> MHHHHHHSEINPAEFEQVNMVLQGFVETSVLPVLELSADESHIEFREHSRNAHTVVWKIISTSYQDELTVSLHITTGKLQIQGRP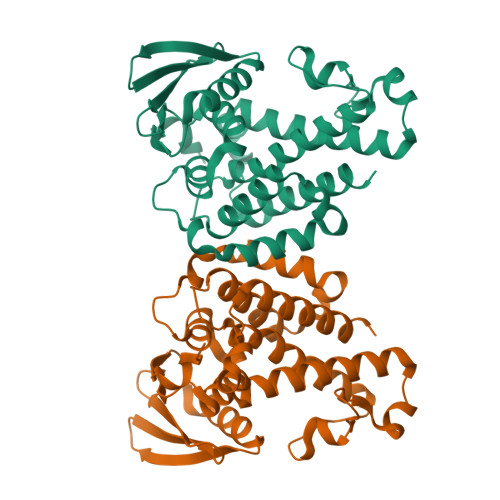LSCYRVFTFNLAALLDLQGLEKVLIRQEDGKANIVQQEVARTYLQTVMADAYPHLHVTAEKLLVSGLCVKLAAPDLPDYCMLLYPELRTIEGVLKSKMSGLGMPVQQPAGFGTYFDKPAAHYILKPQFAATLRPEQINIISTAYTFFNVERHSLFHMETVVDASRMISDMARLMGKATRAWGIIKDLYIV> SECKTGNGKNYRGTMSKTKNGITCQKWSSTSPHRPRFSPATHPSEGLEENYCRNPDNDPQGPWCYTTDPEKRYDY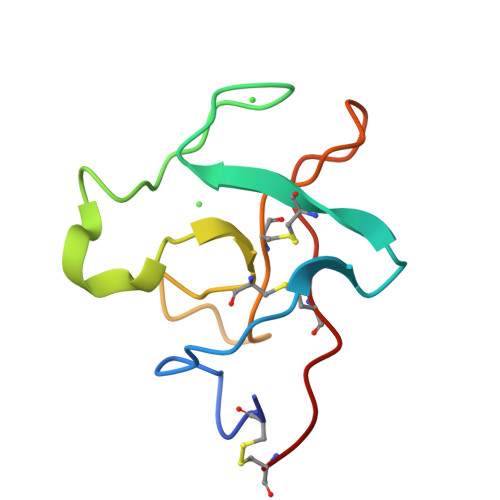CDILECD>MPKQTLDGNTAAAHVAYAMSEVATIYPITPSSPMAEIADEWAAHGRKNIFGKTLQVAEMQSEAGAAGAVHGSLAAGALTTTFTASQGLLLMIPNMYKIAGELLPCVFHVAARALSTHALSIFGDHADVMAARQTGFAMLSSASVQEVMDLALVAHLATLKARVPFVHFFDGFRTSHEVQKIDVIEYEDMAKLVDWDAIRAFRQRALNPEHPHQRGTAQNPDIYFQSREAANPYYLATPGIVAQVMEQVAGLTGRHYHLFDYAGAPDAERVIVSMGSSCEVIEETVNYLVEKGEKVGLIKVRLFRPFSAEHFLKVLPASVKRIAVLDRTKEPGSLGEPLYEDVQTVLAEHGKNILVVGGRYGLGSKEFNPSMVKAVFDNLAATTPKNKFTVGITDDVTHTSLEIKEHIDTSPKGTFRCKFFGLGSDGTVGANKNSIKIIGDHTDMYAQGYFVYDSKKSGGVTISHLRFGKQPIQSAYLIDQADLIACHNPSYVGRYNLLEGIKPGGIFLLNSTWSAEEMDSRLPADMKRTIATKKLKFYNIDAVKIAQEIGLGSRINVIMQTAFFKIANVIPVDEAI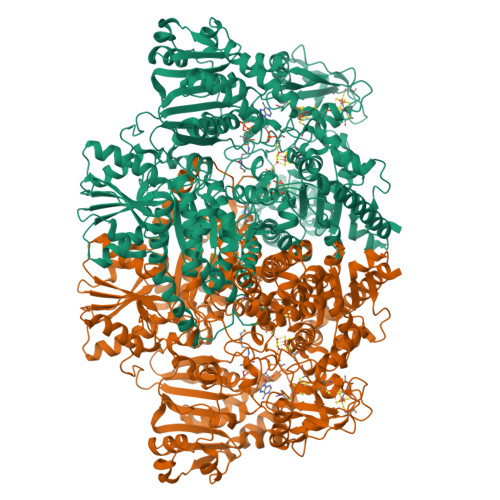KYIKDSIVKTYGKKGDKILNMNFAAVDRALEALEEIKYPASWADAVDEAAATVTEEPEFIQKVLRPINALKGDELPVSTFTPDGVFPVGTTKYEKRGIAVNIPQWQPENCIQCNQCSLVCPHAAIRPYLAKPADLAGAPETFVTKDAIGKEAAGLKFRIQVSPLDCTGCGNCADVCPAKVKALTMVPLEEVTAVEEANYNFAEQLPEVKVNFNPATVKGSQFRQPLLEFSGACAGCGETPYVKLVTQLFGDRMIIANATGCSSIWGGSAPACPYTVNRQGHGPAWASSLFEDNAEFGYGMALAVAKRQDELATAISKALEAPVSAAFKAACEGWLAGKDDADRSREYGDRIKALLPGEISQASGEVKDLLLDIDRQKDYLTKKSIWIIGGDGWAYDIGYGGLDHVLASGANVNVLVLDTEVYSNTGGQSSKATQTGAVARFAAGGKFTKKKDLGLMAMSYGYVYVASVAMGASHSQLMKALIEAEKYDGPSLIIAYAPCINHGINMTYSQREAKKAVEAGYWPLYRYNPQLAQEGKNPFILDYKTPTASFRDFLMGEIRYTSLKKQFPEKAEQLFAKAEADAKARLEQYKKLAEG[3x]> SMRSTKVIHIVGCHAEGEVGDVIVGGVAPPPGKTVWEQSRFIASDETLRNFVLNEPRGGVFRHVNLLVPPKDPRAQMGFIIMEPADTPPMSGSNSICVSTVLLDSGIIPMQEPVTRMVLEAPGGLIEVEAECRNGKAE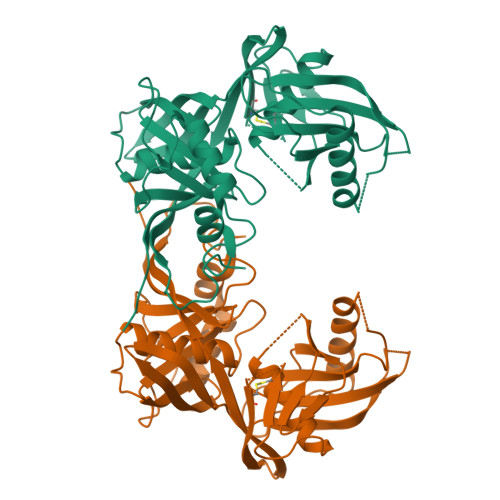RISVRNVPSFADRLNASLEVEGLGTITVDTAYGGDSFVIVDAASIGMKIEPGQARELAEIGVKITKAANEQLGFRHPEKDWNHISFCQITEPVTRDGDILTGVNTVAIRPAKLDRSPTGTGCSARMAVLHAKGQMKVGERFIGKSVLGTEFHCRLDKTLELGGKPAISPIISGRAWVTGTSQLMLDPSDPFPSGYRLSDTWPNMPE> MDPIINGNSANVYLTDSYLKGVISFSECNALGSYIFNGPYLKNDYTNLISRQNPLIEHMNLKKLNITQSLISKYHKGEIKLEEPTYFQSLLMTYKSMTSSEQIATTNLLKKIIRRAIEISDVKVYAILNKLGLKEKDKIKSNNGQDEDNSVITTIIKDDILSAVKDNQSHLKADKNHSTKQKDTIKTTLLKKLMCSMQHPPSWLIHWFNLYTKLNNILTQYRSNEVKNHGFTLIDNQTLSGFQFILNQYGCIVYHKELKRITV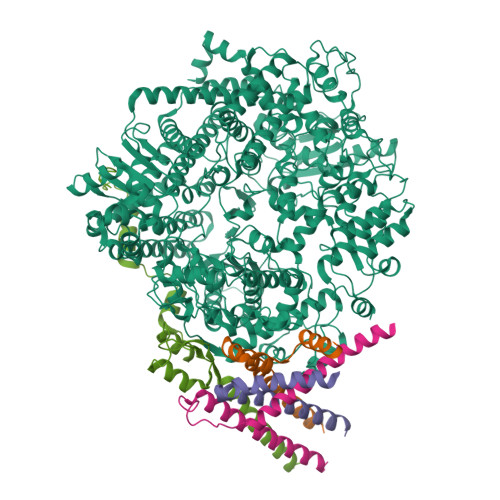TTYNQFLTWKDISLSRLNVCLITWISNCLNTLNKSLGLRCGFNNVILTQLFLYGDCILKLFHNEGFYIIKEVEGFIMSLILNITEEDQFRKRFYNSMLNNITDAANKAQKNLLSRVCHTLLDKTVSDNIINGRWIILLSKFLKLIKLAGDNNLNNLSELYFLFRIFGHPMVDERQAMDAVKINCNETKFYLLSSLSMLRGAFIYRIIKGFVNNYNRWPTLRNAIVLPLRWLTYYKLNTYPSLLELTERDLIVLSGLRFYREFRLPKKVDLEMIINDKAISPPKNLIWTSFPRNYMPSHIQNYIEHEKLKFSESDKSRRVLEYYLRDNKFNECDLYNCVVNQSYLNNPNHVVSLTGKERELSVGRMFAMQPGMFRQVQILAEKMIAENILQFFPESLTRYGDLELQKILELKAGISNKSNRYNDNYNNYISKCSIITDLSKFNQAFRYETSCICSDVLDELHGVQSLFSWLHLTIPHVTIICTYRHAPPYIGDHIVDLNNVDEQSGLYRYHMGGIEGWCQKLWTIEAISLLDLISLKGKFSITALINGDNQSIDISKPIRLMEGQTHAQADYLLALNSLKLLYKEYAGIGHKLKGTETYISRDMQFMSKTIQHNGVYYPASIKKVLRVGPWINTILDDFKVSLESIGSLTQELEYRGESLLCSLIFRNVWLYNQIALQLKNHALCNNKLYLDILKVLKHLKTFFNLDNIDTALTLYMNLPMLFGGGDPNLLYRSFYRRTPDFLTEAIVHSVFILSYYTNHDLKDKLQDLSDDRLNKFLTCIITFDKNPNAEFVTLMRDPQALGSERQAKITSEINRLAVTEVLSTAPNKIFSKSAQHYTTTEIDLNDIMQNIEPTYPHGLRVVYESLPFYKAEKIVNLISGTKSITNILEKTSAIDLTDIDRATEMMRKNITLLIRILPLDCNRDKREILSMENLSITELSKYVRERSWSLSNIVGVTSPSIMYTMDIKYTTSTISSGIIIEKYNVNSLTRGERGPTKPWVGSSTQEKKTMPVYNRQVLTKKQRDQIDLLAKLDWVYASIDNKDEFMEELSIGTLGLTYEKAKKLFPQYLSVNYLHRLTVSSRPCEFPASIPAYRTTNYHFDTSPINRILTEKYGDEDIDIVFQNCISFGLSLMSVVEQFTNVCPNRIILIPKLNEIHLMKPPIFTGDVDIHKLKQVIQKQHMFLPDKISLTQYVELFLSNKTLKSGSHVNSNLILAHKISDYFHNTYILSTNLAGHW;>MEKFAPEFHGEDANNRATKFLESIKGKFTSPKDPKKKDSIISVNSIDIEVTKESPITSNSTIINPTNETDDTAGNKPNYQRKPLVSFKEDPTPSDNPFSKLYKETIETFDNNEEESSYSYEEINDQTNDNITARLDRIDEKLSEILGMLHTLVVASAGPTSARDGIRDAMVGLREEMIEKIRTEALMTNDRLEAMARLRNEESEKMAKDTSDEVSLNPTSEKLNNLLEGNDSDNDLSLEDF[4x]>GGGRNPPEGASEEGGAADSDVDAFFRTGSFRNDGLKASDVLPILKEKVAFVSGGRDKRGGPILTFPARSNHDRIRQEDLRKLVTYLASVPSEDVCKRGFTVIIDMRGSKWDLIKPLLKTLQEAFPAEIHVALIIKPDNFWQKQKTNFGSSKFIFETSMVSVEGLTKLVDPSQLTEEFDGSLDYNHEEWIELRLSL[8x]

The neuronal RhoGEF Kalirin, a central regulator of cytoskeletal dynamics, contains a Sec14 domain (KalbSec14) followed by multiple spectrin-like repeats and catalytic domains. The N-terminal CRAL_TRIO domain of Kalirin is followed by nine SRs and a variable number of RhoGEF (consisting of DH and PH domains), SH3 and protein kinase domains. Kal7, the major isoform expressed in the adult brain, supports the formation and function of excitatory synapses. KalbSec14 adopts a closed conformation, sealing off the canonical ligand entry site, and instead employs a surface groove to bind a limited set of lysophospholipids.

We obtained diffraction-quality crystals of KalbSec14, a construct consisting of the Ex1B front peptide (residues 1–25), the putative CRAL-TRIO domain (residues 26–182) and a part of the predicted A-helix (residues 183–192) of the first SR. The X-ray crystal structure of KalbSec14 was determined at 1.89-Å resolution by single-wavelength anomalous dispersion using a selenomethionine derivative and refined to an R factor of 19.5% and an Rfree value of 21.8%. The asymmetric unit contains eight nearly identical protein monomers, with an overall root mean square deviation (rmsd) of 0.8 Å for 175 Cα atoms. The central β sheet is composed of five strands (S1–S5), with S1 the only antiparallel strand, and is flanked by six α helices (H1–H6) and a 310 helix (H7) on one side and by two α helices, H8 and H9, on the other. An N-terminal 10-amino-acid extension (residues 18–27) upstream of the H1 helix projects ~18 Å away from the αβα core, confirming the notion that the Sec14 domain of Kalirin lacks the CRAL_TRIO_N domain found in many stand-alone Sec14 proteins. As such, the interaction of the C-terminal H9 helix, which is part of the first SR, with the central αβα fold buries 441 Å2 of solvent-accessible surface area. Unexpectedly, KalbSec14 has only several small, discontinuous hydrophobic pockets (~100 Å3 each) in the center of its αβα fold, none of which is large enough to accommodate even a single phospholipid molecule. Moreover, the 310 helix H7, along with an extended loop, is positioned across any potential openings into these internal pockets, mimicking the closed conformation of the so-called mobile gate as often observed for holo-forms of other Sec14 proteins. Nevertheless, an elongated groove is present on the surface of KalbSec14, directly above the S2 and S3 strands. Our NMR CSP data and mutagenesis studies demonstrate that the residues lining a distinct surface groove of the Kalirin Sec14 domain are responsible for its interaction with selected detergents and LPC lipids.> DLSASVPTRPAEPERKTLADYGGYPSALDAVKQKNDAAVAAYLENAGDSAMAENVRNEWLKSLGARRQWTLFAQEYAKLEPAGRAQEVECYADSSRNDYTRAAELVKNTGKLPSGCTKLLEQAAASGLLDGNDAWRRVRGLLAGRQTTDARNLAAALGSPFDGGTQGSREYALLNVIGKEARKSPNAAALLSEMESGLSLEQRSFAWGVLGHYQSQNLNVPAALDYYGKVADRRQLTDDQIEWYARAALRARRWDELASVISHMPEKLQKSPTWLYWLARSRAATGNTQEAEKLYKQAAATGRNFYAVLAGEELGRKIDTRNNVPDAGKNSVRRMAEDGAVKRALVLFQNSQSAGDAKMRRQAQAEWRFATRGFDEDKLLTAAQTAFDHGFYDMAVNSAERTDRKLNYTLRYISPFKDTVIRHAQNVNVDPAWVYGLIRQESRFVIGAQSRVGAQGLMQVMPATAREIAGKIGMDAAQLYTADGNIRMGTWYMADTKRRLQNNEVLATAGYNAGP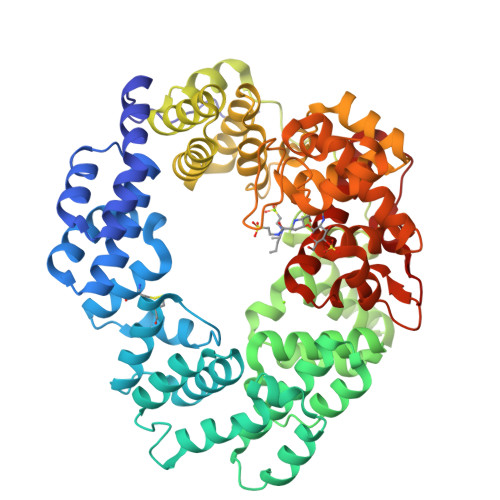GRARRWQADTPLEGAVYAETIPFSETRDYVKKVMANAAYYAALFGAPHIPLKQRMGIVPAR> MKEQLEDVLDTLTDREENVL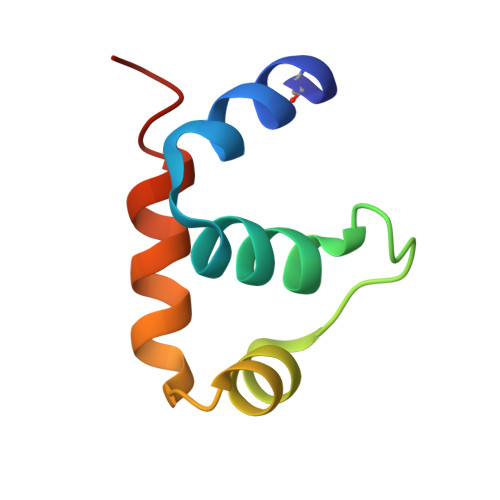RLRFGLDDGRTRTLEEVGKVFGVTRERIRQIEAKALRKLRHP phosphinate 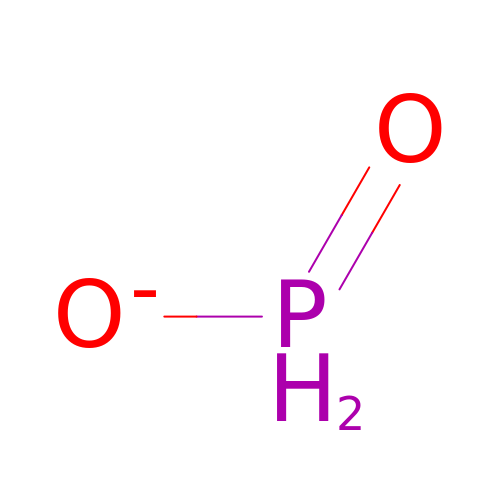| H2 O2 P | ACVYVLVWPXVTIT-UHFFFAOYSA-M>[2x]GHMNVKRRTHNVLERQRRNELKRSFFA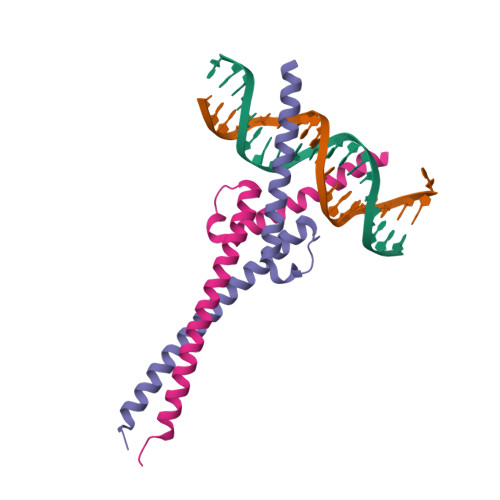LRDQIPELENNEKAPKVVILKKATAYILSVQAEEQKLISEEDLLRKRREQLKHKLEQLGGC;>[2x]DKRAHHNALERKRRDHIKDSFHSLRDSVPSLQGEKASRAQILDKATEYIQYMRRKNHTHQQDIDDLKRQNALLEQQVRALGGC1-benzyl-3-(2-chloropyridin-4-yl)urea 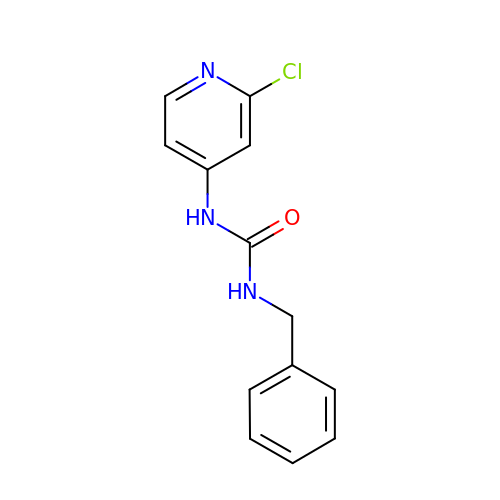| C13 H12 Cl N3 O | XDVQQOIDSVMNNN-UHFFFAOYSA-N> AYACSFPPSEIPGSKECLAEALQKHQGFKKK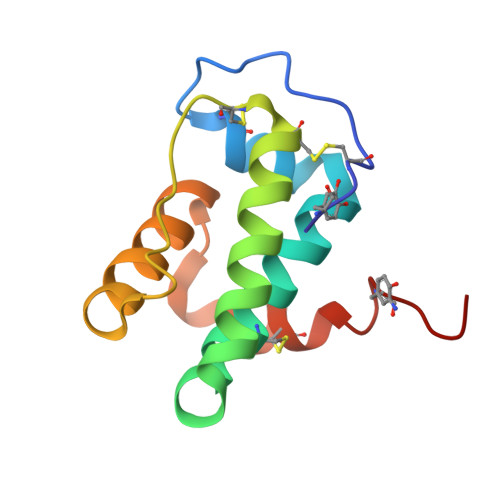SYALICAYLNYKEDAENYERAAEDFDSAVKCTGCKEGVDLHEGNPELIEEGFEKFLASLKIDRKALGSLCTLFQKLYAIPHN>[12x]RLIHVSRCEMGTSTHRCWPRPCDTSSDEPISFWPPFENTPNVIVSFGMLD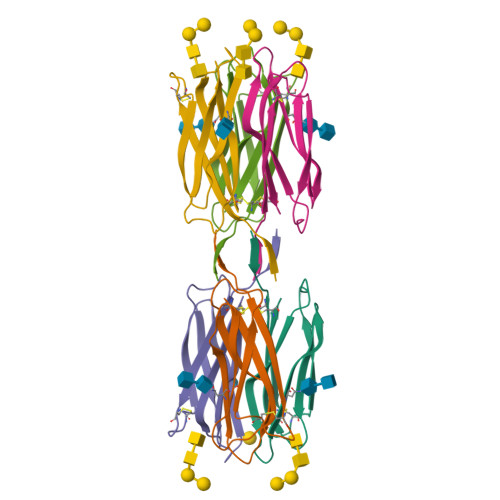VDNSNNLRVNSSADDVTVGGFTLHYNSWYTTTVWNYKLIWIACD>MEGESSISIGYAQSRVKEDGYKLDKNPRGFNLKYRYEFNNDWGVIGSFAQTRRGFEESVDGFKLIDGDFKYYSVTAGPVFRINEYVSLYGLLGAGHGKAKFSSIFGQSESRSKTSLAYGAGLQFNPHPNFVI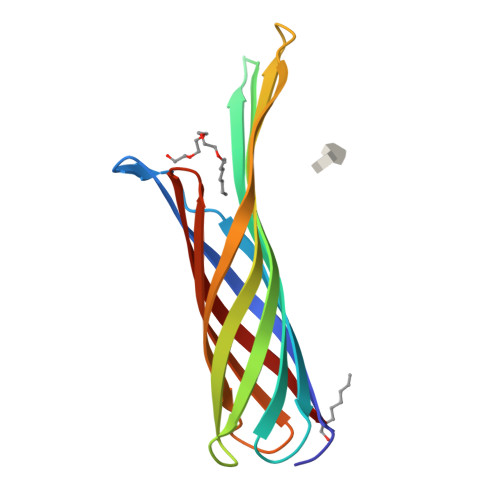DASYEYSKLDDVKVGTWMLGAGYRF[2x]>[2x]MSAVMATYLLHDETDIRKKAEGIA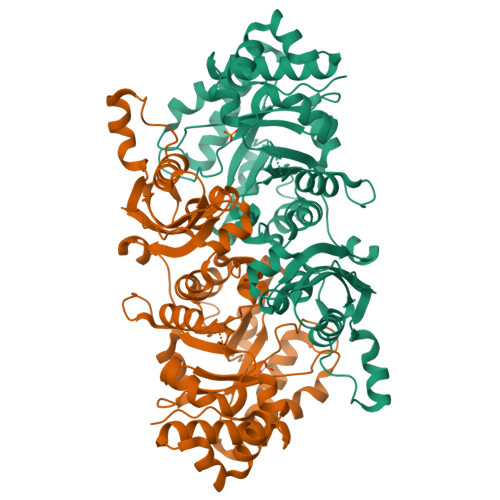LGLTIGTWTDLPALEQEQLRKHKGEVVAIEELGESERVNAYFGKRLKRAIVKIAYPTVNFSADLPALLVTTFGKLSLDGEVRLLDLEFPDEWKRQFPGPRFGIDGIRDRVGVHNRPLLMSIFKGMIGRDLAYLTPELKKQALGGVDLVKDDEILFDSELLPFEKRITEGKAALQEVYEQTGKRTLYAVNLTGKTFALKDKAKRAAELGADVLLFNVFAYGLDVLQALREDEEIAVPIMAHPVFSGAVTPSEFYGVAPSLWLGKLLRLAGADFVLFPSPYGSVASEREQALGIARALTDDQEPFARAFPVPSAGIHPGLVPLIIRDFGLDTIVNAGGGIHGHPHGAIGGGRAFRAAIDAVLAGRPLRAAAAENEALQKAIDRWGVVEVEA3-methoxy-4,5-bis(oxidanyl)benzoic acid | C8 H8 O5 | 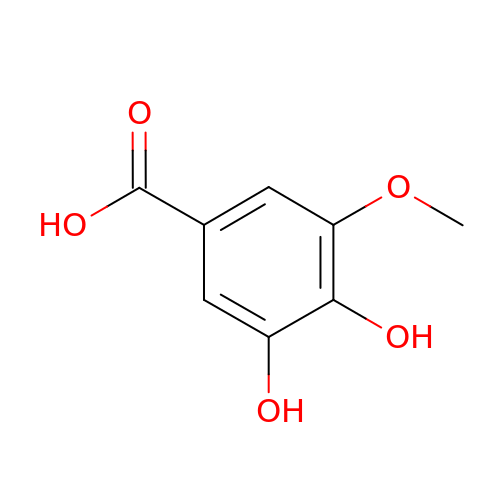KWCCUYSXAYTNKA-UHFFFAOYSA-N>[2x]GSKLETKQRSPVEIIDDVKDEIQKRELIYDALHKLNSPNEEKEYFNIHAWDVWHDMISVRALTVDSDVEIYKVLKAMSSAKITQATTGYKGTQLKAMFSLDGPQIQNVVFKPKRYSRNKIILGTPYEGYDRHNAEIAAFHLDRLLGFYRAPPVVGRYINLAAEVLPVAAKKLATTFIKDKDENLCFYGKCLYCNRKEPACASNVTMEGALILWLPEKWPVLKLPHPWRRTYNKKMAKWETDSHYCESVVIKEPYTKGPRLLDLIDTSIFDFLIGNADRHHYEYIENENGSMVIHLDNAKSFGNPFVDEKSILSPLVQCCRLRSSTYNRLKIATSNENSLSVLLDKRLSIDPIYPILTSDHLLALDRRLLLVQDAVEKCFKEKNKENVIIEDHL

The Fam20 proteins are recently identified kinases that regulate essential cellular processes by phosphorylating proteins and proteoglycans. The human genome encodes three Fam20 paralogs: Fam20A, Fam20B, and Fam20C13. Remarkably, each has a distinct biochemical activity. Here, we use a combination of structural biology, biochemistry, and phylogenetics to elucidate the molecular functions and evolutionary relationships of the three Fam20 kinases.

In contrast, the single Fam20 proteins in basal animals such as sponge (Amphimedon queenslandica, aqFam20) and hydra (Hydra magnipapillata, hmFam20) are apparently Fam20B-like because they exhibit robust activity for the Galβ1-4Xylβ1 disaccharide (Gal-Xyl hereafter), and do not phosphorylate protein substrates such as OPN, casein, and enamelin. Although human Fam20B can be purified to homogeneity, it failed to crystallize despite extensive trials. hmFam20 crystallized readily, but the initial crystals diffracted poorly. Treatment of the purified hmFam20 with endoglycosidase F3 to remove the majority of the N-linked glycans significantly improved crystal quality and diffraction. The hmFam20 structure was subsequently determined at 2.2 Å resolution. The overall structure of hmFam20 resembles that of Fam20C, and can be superimposed onto ceFam20 with a root-mean-square deviation of 1.5 Å over 342 aligned Cα atoms. There are four disulfide bonds in hmFam20 (Cys207-Cys222, Cys212-Cys215, Cys267-Cys340, Cys341-Cys400), which all align with the four disulfide bonds in Fam20C. The hmFam20 structure enabled us to consider how Fam20C may have emerged in higher animals. Inspection of the hmFam20 structure (Fam20B-like) and the ceFam20 structure (Fam20C-like) reveals three regions in Fam20C that lead to a change in substrate preference. The single Fam20 protein in hydra is also Fam20B-like, which likely plays a similar role in regulating proteoglycan synthesis as its ortholog in higher animals.>MSLSVPFEYTPIAQSVLDECEHLDTASLSDALDSLGIDGGLPGIASQVPGTRCVGIAFTVQYQPVDASEGFRGAANYIDQVPSGSVIVSSNSGRHDCTVWGDIMTHFALANGIKGTVIDGVAR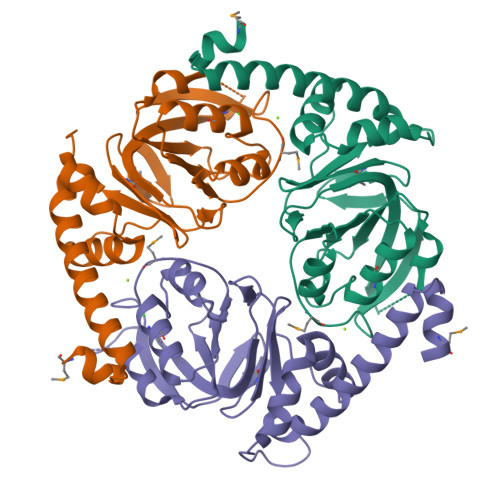DIDTVINCNYPLFSRGRFMQSAKNRTQLKAVQVPLVIDGITIQPGDLMVCDGSGCVVVPQQLAAEVVLRARAVEQTERRIIEAISSGSTLEQARMTYRYDQPWLSEAEHGGTQEGHHHHHH[3x]> GAMGSNLKDMEQNSAKAVVLLKAMANERRLQILCMLHNQELSVGELCAKLQLSQSALSQHLAWLR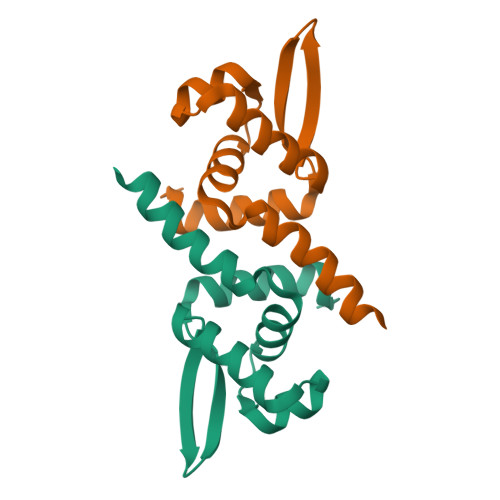RDGLVTTRKEAQTVYYTLKSEEVKAMIKLLHSLYCEE> MEELKSYYKRVAKYYSAAALLYWDMQTYMPKDAGPYRAEVLSEIGTYAFKQITDDALGKLLETAQPQSEIDEKLVYVGKKEYYKYKKVPPELFQEIMITSTMLEQKWEIAKPRGDFEEVRPLLEKIVDLSRKYADILGYEGEPYNALLDLYEPGMKAEEVDQIFSKVRDFIVEVLEKIERLPKSEDPFNREIGVDKQKEFSNWLLHYLKYDFTKGRLDVSAHPFTNPIGLNDVRITTRYIVNDIRNSIYSTIHEFGHALYALSIPTEFYGLPIGSSASYGFDESQSRFWENVVGRSLAFWKGIYSKFIEIVPEMRGYSVEELWRAVNRVQRSFIRTEADEVTYNLHIIIRFEIER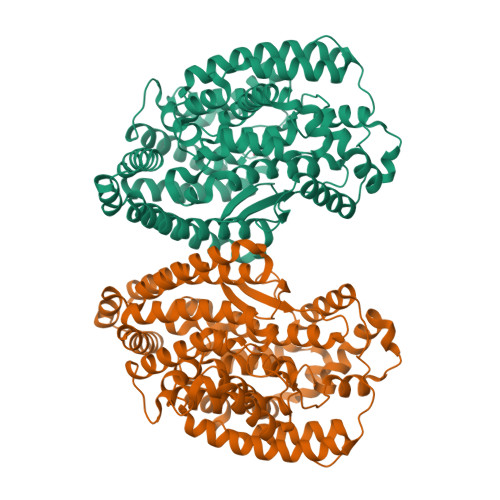ELINGELSVKDVPDKWNELYKKYLGLDVPNNTLGCMQDPHWFGGNFGYFPTYALGNLYAAQIFEKLKEEINFEEVVSAGNFEIIKNFLKEKIHSKGKMYEPSDLIKIVTGKPLSYESFVRYIKDKYSKVYEIEL N-{(1S,2S)-1-BENZYL-2-HYDROXY-2-[(4S)-1,2,2-TRIMETHYL-5-OXOIMIDAZOLIDIN-4-YL]ETHYL}-N'-[(1R)-1-(4-FLUOROPHENYL)ETHYL]-5-[METHYL(METHYLSULFONYL)AMINO]ISOPHTHALAMIDE | 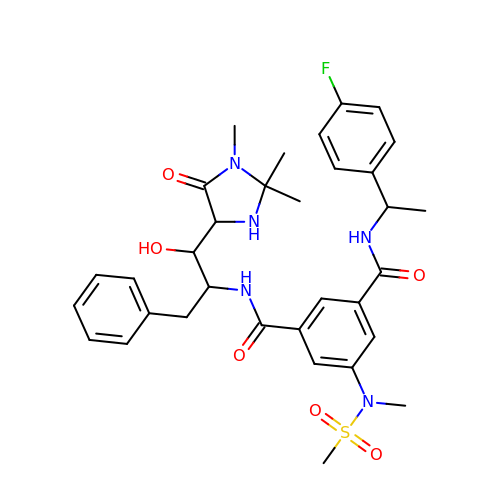C33 H40 F N5 O6 S | YNXGIROKYOHHJW-UFAZYNLISA-N> GSPALDTGTTEEDRLKIDVIDWLVFDPAQRAEALKQGNAIMRKFLASKKHEAAKEVFVKIPQDSIAEIYNQCEEQGMESPLPAEDDNAIREHLCIRAYLEAHETFNEWFKHMNSVPQKPALIPQPTFTEKVAHEHKEKKYEMDFGIWKGHLDALTADVKEKMYNVLLFVDGGWMVDVREDAKEDHERTHQMVLLRKLCLPMLCFLLHTILHSTGQYQECLQLADMVSSERHKLYLVFSKEELRKLLQKLRESSLMLLDQGLDPLGYEIQLSGRIVTD;> GSHMDKIKLLKAAFLQYCRKDLGHAQMVVDELFSSHSDLDSDSELDRAVTQISVD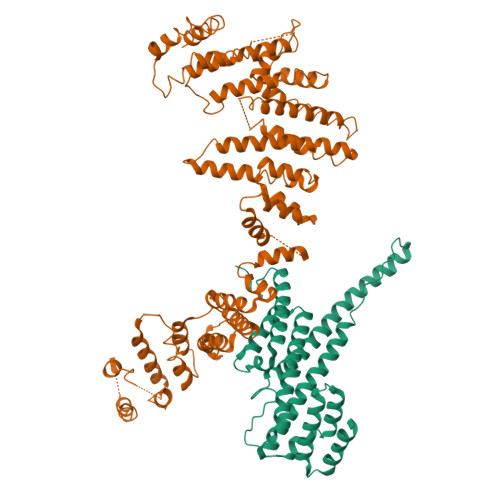LMDDYPASDPRWAESVPEEAPGFSNTSLIILHQLEDKMKAHSFLMDFIHQVGLFGRLGSFPVRGTPMATRLLLCEHAEKLSAAIVLKNHHSRLSDLVNTAILIALNKREYEIPSNLTPADVFFREVSQVDTICECLLEHEEQVLRDAPMDSIEWAEVVINVNNILKDMLQAASHYRQNRNSLYRREESLEKEPEYVPWTATSGPGGIRTVIIRQHEIVLKVAYPQADSNLRNIVTEQLVALIDCFLDGYVSQLKSVDKSSNRERYDNLEMEYLQKRSDLLSPLLSLGQYLWAASLAEKYCDFDILVQMCEQTDNQSRLQRYMTQFADQNFSDFLFRWYLEKGKRGKLLSQPISQHGQLANFLQAHEHLSWLHEINSQELEKAHATLLGLANMETRYFAKKKTLLGLSKLAALASDFSEDMLQEKIEEMAEQERFLLHQETLPEQLLAEKQLNLSAMPVLTAPQLIGLYICEENRRANEYDFKKALDLLEYIDEEEDININDLKLEILCKALQRDNWSSSDGKDDPIEVSKDSIFVKILQKLLKDGIQLSEYLPEVKDLLQADQLGSLKSNPYFEFVLKANYEYYVQGQI>AEKLQTTLRVGTYF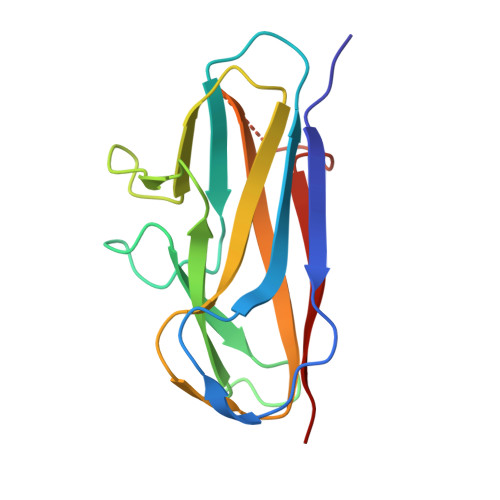RAGHVPDGMVLAQGWVTYHGSHSGFRVWSDEQKAGNTPTVLLLSGQQDPRHHIQVRLEGEGWQPDTVSGRGAILRTAADNASFSVVVDGNQEVPADTWTLDFKACALAQEDTDNKQGSFLPNSEQQKSVDIVFSS[2x]> MDDEDNKCDCPPPGLPLWMGTFADLMSLLMCFFVLLLSFSEMDVLKFKQIAGSMKFAFGVQNQLEVKDIPKGTSIIAQEFRPGRPEPTPIDVIMQQTMDITQQTLEFHEGESDRAGGTKRDEGKLTGGQSPATSTQNNESAEADMQQQQSKEMSQEMETLMESIKKALEREIEQGAIEVENLGQQIVIRMREKGAFPEGSAFLQPKFRPLVRQIAELVKDVPGIVRVSGHTDNRPLDSELYRSNWD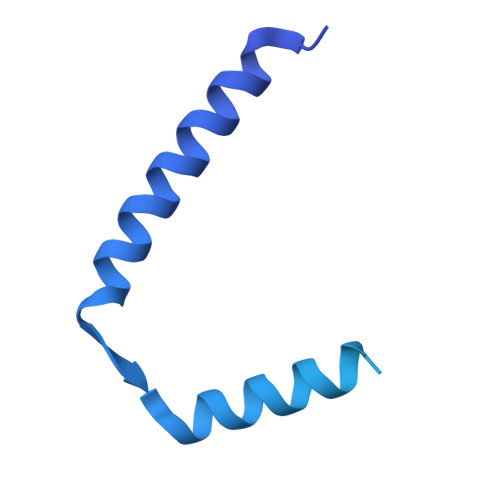LSSQRAVSVAQEMEKVRGFSHQRLRVRGMADTEPLLPNDSDDNRALNRRVEISIMQGEPLYSEEVPVIQHHHHHH> MTLYMGPNTGLLINGLPGEGHYSDLIRMWRWDDFLRQPVVKGRVATLPTTGQAEGDTYIFTGSGSNQNRLARWWATGATTAIWEYMPPRLGWRVQVANETTPSGQVKTYEYSGTAWVELVGGMSDAPSDGKAYARESGAWTELGSAAKSALNVLPFMNLMPDMGRFAGTAANPLATMFTTSWTPSSFLNGWNGATVADGGKFAFDNSTNGGAGPALNARVQALLAAMGRTWTSVSRYGVEFFTAVLTAGSQTTTGSAGADGVTRYLCCSNGSKTVFNAGGWATVVMWLRVESGSAHISSAPYTTHRLWINGAVAAPGVVLPANQWVHLRFSMQSYNGYDNACPYIYASAGAQIAFACPAWFGGLVDPGI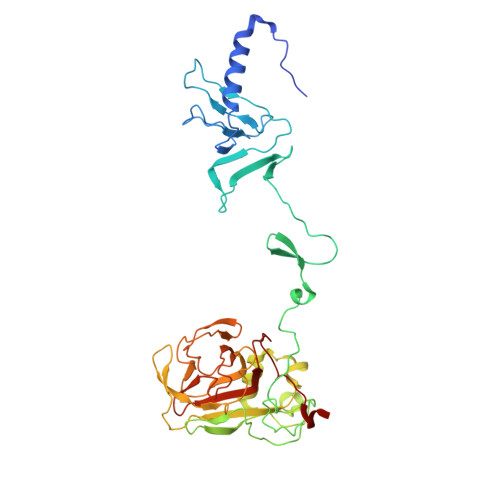HVAPILTINGASA> RFRARYRWRRKNGITNLRLTRQVELWVPKDAANASFYVNHYTFDLDDFIPAGTQLNSSPLPFKYYRIRKVKVEFQPRLPITSP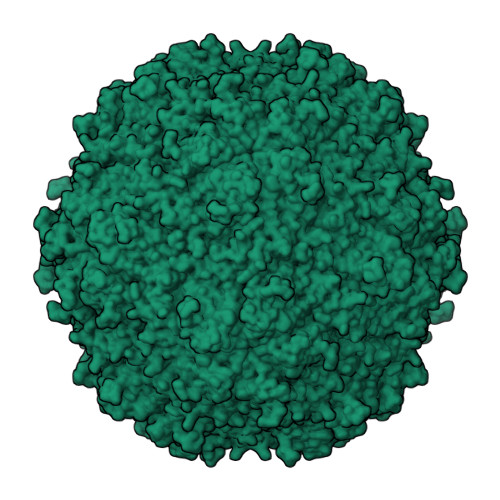FRGYGSTVPILDGAFVTPATGESDPIWDPYINFSGRHVIRTPAWYHKRYFTPKPLIDGNTGFFQPNNKQNALWFPNKQGQNIQWSGLGFAMQKGNEAYNYQVRFTLYVQFREFDLFNN>MHHHHHHMARIRAMKRHYEAVVIGGGIIGSAIAYYLAKENKNTALFESGTMGGRTTSAAAGMLSAHRECEERDAFFDFAMHSQRLYKGLGEELYALSGVDIRQHNGGMFKLAFSEEDVLQLRQMDDLDSVSWYSKEEVLEKEPYASGDIFGASFIQDDVHVEPYFVCKAYVKAAK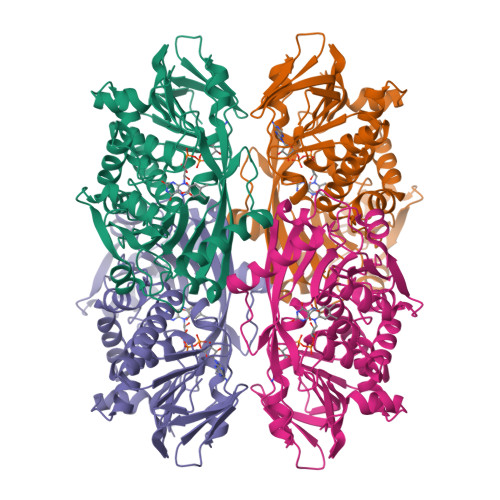MLGAEIFEHTPVLHVERDGEALFIKTPSGDVWANHVVVASGVWSGMFFKQLGLNNAFLPVKGECLSVWNDDIPLTKTLYHDACYIVPRKSGRLVVGATMKPGDWSETPDLGGLESVMKKAKTMLPAIQNMKVDRFWAGLRPGTKDGKPYIGRHPEDSRILFAAGHFRNGILLAPATGALISDLIMNKEVNQDWLHAFRIDRKEAVQI[4x]>[4x]MEIAFLLNGETRRVRIEDPTQSLLEWLRAEGLTGTKEGCNEGDCGACTVMIRDAAGSRAVNACLMMLPQIA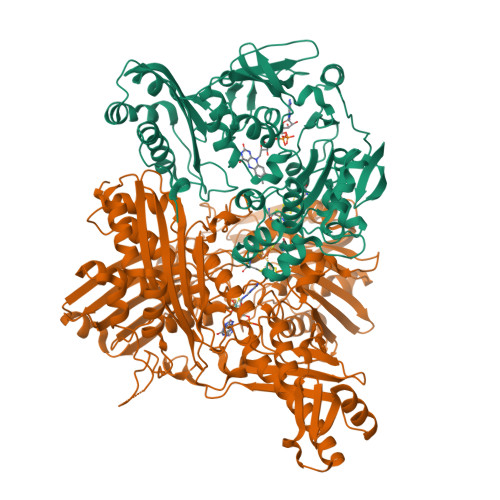GKALRTIEGIAAPDGRLHPVQQAMIDHHGSQCGFCTPGFIVSMAAAHDRDRKDYDDLLAGNLCRCTGYAPILRAAEAAAGEPPADWLQADAAFTLAQLSSGVRGQTAPAFLPETSDALADWYLAHPEATLIAGGTDVSLWVTKALRDLPEVAFLSHCKDLAQIRETPDGYGIGAGVTIAALRAFAEGPHPALAGLLRRFASEQVRQVATIGGNIANGSPIGDGPPALIAMGASLTLRRGQERRRMPLEDFFLEYRKQDRRPGEFVESVTLPKSAPGLRCYKLSKRFDQDISAVCGCLNLTLKGSKIETARIAFGGMAGVPKRAAAFEAALIGQDFREDTIAAALPLLAQDFTPLSDMRASAAYRMNAAQAMALRYVRELSGEAVAVLEVMP;>[4x]MSVGKPLPHDSARAHVTGQARYLDDLPCPANTLHLAFGLSTEASAAITGLDLEPVRESPGVIAVFTAADLPHDNDASPAPSPEPVLATGEVHFVGQPIFLVAATSHRAARIAARKARITYAPRPAILTLDQALAADSRFEGGPVIWARGDVETALAGAAHLAEGCFEIGGQEHFYLEGQAALALPAEGGVVIHCSSQHPSEIQHKVAHALGLAFHDVRVEMRRMGGGFGGKESQGNHLAIACAVAARATGRPCKMRYDRDDDMVITGKRHDFRIRYRIGADASGKLLGADFVHLARCGWSADLSLPVCDRAMLHADGSYFVPALRIESHRLRTNTQSNTAFRGFGGPQGALGMERAIEHLARGMGRDPAELRALNFYDPPERGGLSAPPSPPEPIATKKTQTTHYGQEVADCVLGELVTRLQKSANFTTRRAEIAAWNSTNRTLARGIALSPVKFGISFTLTHLNQAGALVQIYTDGSVALNHGGTEMGQGLHAKMVQVAAAVLGIDPVQVRITATDTSKVPNTSATAASSGADMNGMAVKDACETLRGRLAGFVAAREGCAARDVIFDAGQVQASGKSWRFAEIVAAAYMARISLSATGFYATPKLSWDRLRGQGRPFLYFAYGAAITEVVIDRLTGENRILRTDILHDAGASLNPALDIGQIEGAYVQGAGWLTTEELVWDHCGRLMTHAPSTYKIPAFSDRPRIFNVALWDQPNREETIFRSKAVGEPPFLLGISAFLALHDACAACGPHWPDLQAPATPEAVLAAVRRAEGRA>[8x]MLARHGPRYGGSVNGHSDDSSGDAKQAAPTLYIFPHAGGTAKDYVAFSREFSADVKRIAVQYPGQHDRSGLPPLESIPTLADEIFAMMKPSARIDDPVAFFGHSMGGMLAFEVA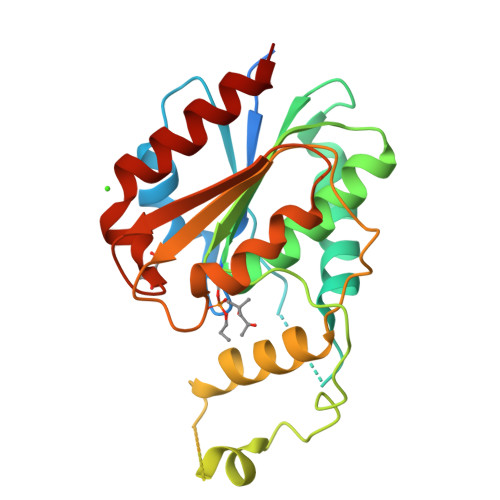LRYQSAGHRVLAFFVSACSAPGHIRYKQLQDLSDREMLDLFTRMTGMNPDFFTDDEFFVGALPTLRAVRAIAGYSCPPETKLSCPIYAFIGDKDWIATQDDMDPWRDRTTEEFSIRVFPGDHFYLNDNLPELVSDIEDKTLQWHDRA> MKIVPPKPFFFEAGERAVLLLHGFTGNSADVRMLGRFLESKGYTCHAPIYSGHGVPPEALTRFGPEAWWQDVMNGYEFLKNKGYEKIAVAGLSLGGVFSLKLGYTVPIEGIVTMCAPMYIKSEETMYEGV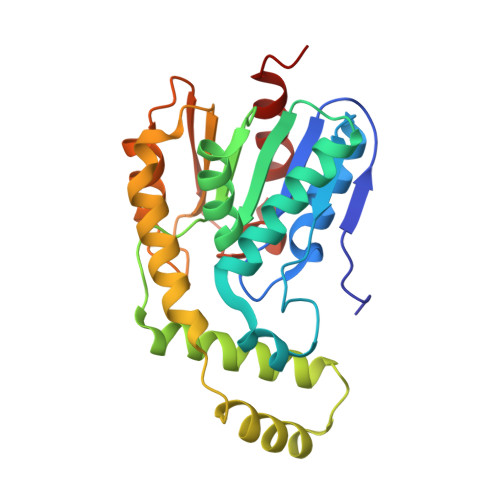LEYAREYKKREGKSEEQIEQEMEKFKQTPMLTLKALQELIADVRDHLDLIYAPTFVVQARHDEMINPDSANIIYNEIESPVKQIKWYEQSGHVITLDQEKDQLHEDIYAFLESLDWLE>AKHLFTSESVSEGHPDKIADQISDAVLDAILEQDPKARVACETYVKTGMVLVGGEITTSAWVDIEEITRNTVREIGYVHSDMGFDANSCAVLSAIGKQSPDINQGVDRADPLEQGAGDQGLMFGYATNETDVLMPAPITYAHRLVQRQAEVRKNGTLPWLRPDAKSQVTFQYDDGKIVGIDAVVLSTQHSEEIDQKSLQEAVMEEIIKPILPAEWLTSATKFFINPTGRFVIGGPMGDCGLTGRKIIVDTYGGMARHGGGAFSGKDPSKVDRSAAYAARYVAKNIVAAGLADRCEIQVSYAIGVAEPTSIMVETFGTEKVPSEQLTLLVREFFDLRPYGLIQMLDLLHPIYKETAAYGHFGREHFPWEKTDKAQL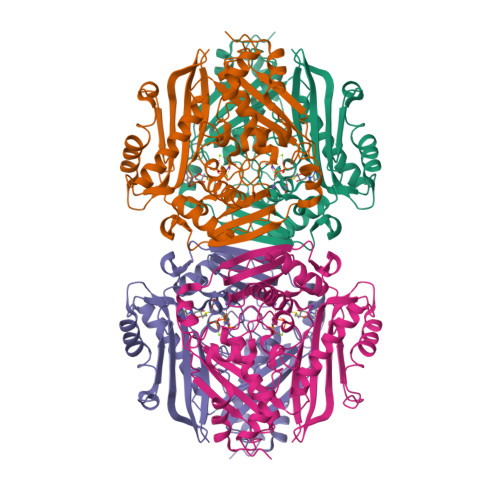LRDAAGLK[4x]> GSKLIHVPKEDNSKEVTLDSLLEEGVLDKEIHKAITRMEFPGLTPVQQKTIKPILSSEDHDVIARAKTGTGKTFAFLIPIFQHLINTKFDSQYMVKAVIVAPTRDLALQIEAEVKKIHDMNYGLKKYACVSLVGGTDFRAAMNKMNKLRPNIVIATPGRLIDVLEKYSNKFFRFVDYKVLDEADRLLEIGFRDDLETISGILNEKNSKSADNIKTLLFSATLDDKVQKLANNIMNKKECLFLDTVDKNEPEAHERIDQSVVISEKFANSIFAAVEHIKKQIKERDSNYKAIIFAPTVKFTSFLCSILKNEFKKDLPILEFHGKITQNKRTSLVKRFKKDESGILVCTDVGARGMDFPNVHEVLQIGVPSELANYIHRIGRTARSGKEGSSVLFICKDELPFVRELEDAKNIVIAKQEKYEPSEEIKSEVLEAVTEEPEDISDIVISLISSYRSCIKEYRFSERRILPEIASTYGVLLNDPQLKIPVSRRFLDKLGLSRSPIGKAMFEIR

(D) Model for RNA duplex binding and unwinding by Mss116. of short duplexes bound to D2 by excluding one RNA strand and bending the other. hydrolysis leads to core re-opening and enzyme turnover in DEAD-box proteins and perhaps other SF1 and SF2 helicases. ‘clamp’ ssRNA and form a highly stable closed-state complex.

A10-RNA + NDP-BeFx, N = A, C, G, or U. However, each base interacts differently in the ATP-binding pocket. H-bonding interactions between the Q-motif and adenine base. the adenine base that further stabilize the closed-state complex. significantly more stable and long-lived with ssRNA than with ssDNA. Ic in D1 with 2′-OH groups of ssRNA in the closed state.> DDKAMAGNFWQSSHYLQWILDKQDLLKERQKDLKFLSEEEYWKLQIFFTNVIQALGEHLKLRQQVIATATVYFKRFYARYSLKSIDPVLMAPTCVFLASKVEEFGVVSNTRLIAAATSVLKTRFSYAFPKEFPYRMNHILECEFYLLELMDCCLIVYHPYRPLLQYVQDMGQEDMLLPLAWRIVNDTYRTDLCLLYPPFMIALACLHVACVVQQKDARQWFAELSVDMEKILEIIRVILKLYEQWKNFDERKEMATILSKMPKPKPPPNS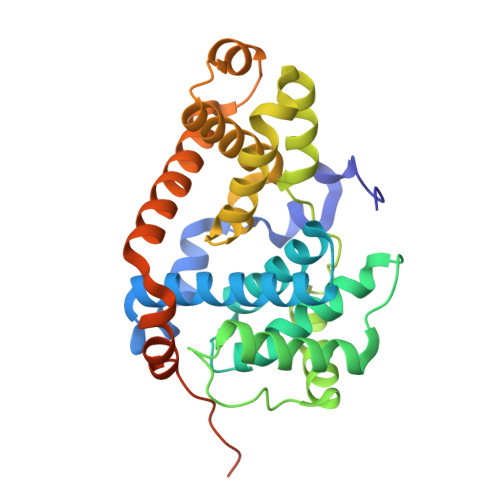EGEQGPNGSQNSSYSQS>GQDMVSPPPPIADEPLTVNTGIYLIECYSLDDKAETFKVNAFLSLSWKDRRLAFDPVRSGVRVKTYEPEAIWIPEIRFVNVENARDADVVDISVSPDGTVQYLERFSARVLSPLDFRRYPFDSQTLHIYLIVRSVDTRNIVLA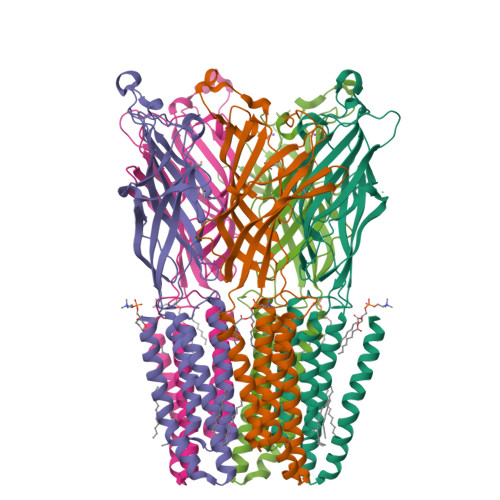VDLEKVGKNDDVFLTGWDIESFTAVVKPANFALEDRLESKLDYQLRISRQYFSYIPNIILPMLFILFISWTAFWSTSYEANVTLVVSTLIAHIAFNILVETNLPKTPYMTYTGAIIFMIYLFYFVAVIEVTVQQYLKVESQPARAASITRASRIAFPVVFLLANIILAFLFFGF[5x]> ETGQVAASPSINVALKAAFPSPPYLVELLETAASDNTTIYYSLLDRIAKGHFAEATTDKALYEKFLEVLRDDGHMDPEALSAFKLALSLRTATPRVEAHYQYYTATVEPSLSGTQEGCDQWFLIDGEQYCSPTLDTSHGKVKGEDQLRTLPFDRKFGVGSRDVILYADITSKSFAPFHEVAMDLAKKGKASYRVRYRRSPSHSRESLSVNGYGVELVLKRTDYIVIDDRDTGAAAKPAEENDQKPLVGHETVLDDGEEIADIKPLEKSELAALGMKAASFVMQSEKPFEALLKLTQDFPKYSNSLGSQNVSAEFEAEHRGNREVFLPEGSNVLWLNGLHLIDRQIQPFGLVDLLTRERKLIKSVLDLGLTGQQAVDLLGHAEVAHAKSGDDEPRRFDWRDDIEEGQVIIWLNNLEKDKRYKSFSPSIWVLIHHFGHGLPQIRRDVFNLVVPVDLTKADDVKIVVEGLLSFVKRLIPVRFGFVPLTPTGQAIDQAKVVYYLLENYGLAAATAYLEKSYEEQSTGQPNERIFNEVIKDKSLRPDGVELSFKDIFISEKHEKQIHLSKHWVERLRAGGDVPTVFFDGFPIPREDNWLRVMNHRLMQDLQALQQAGYFGMLNESMWLPGFFLEKALSRRNTLIFPEDKNELTVLNVNKIYIENHDLMSKVPVIEASKESTRDDWAALTVVADLDDIEGQELVYYALRFRKSNDGVRLDIVHNPKDTSRSPSVLAQRLKSREDKLLDFTRFLDLETALETGEFEPDVAYDASLANFLASSNMKAGDNFVILNGRVLGPITSADDFKKEDFEVFLQAERRTRILPVYKALEDLGLDDKVSGPLSAAKLTSVT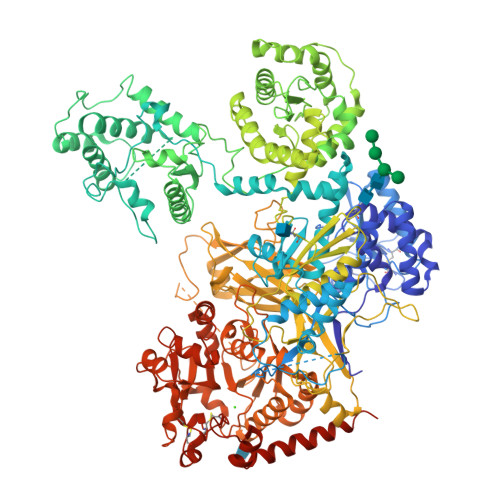ALSTISDLPQGIFDNAPTVRTTLFKQWNSTYTSFEVGDASTATIFFVAVINPASEIGQRWVAVLKVLSELEGVHLRVFLNPTVMIEELPVKRFYRYVLSSSPSFDESGKVKALSARFTGVPRETLLVVGMDVPPAWLVTSKVAVDDLDNLRIKDIKAKRGTEHVEAIYELEHILIEGHSREIPGAHAPRGVQLVLETENNPHFADTIIMANLGYFQFKANPGVYNIRLKEGRSSEIFTLESVGAKGWGPIPGDDNTEVVLMDFQGTTLYPRLRRKPGMEEEDVLEPSTKSGEESGSGARNLVSRGIKFAEGLLGRGNKAAEATKSVSKTEHAEINIFSVASGHLYERMLNIMMASVMHHTNHTVKFWFIEQFLSPSFKDFIPHMAAEYGFKYEMVTYKWPHWLRQQKEKQREIWGYKILFLDVLFPLSLDKVIFVDADQIVRTDMYDLVEHPLDGAPYGFAPMCDSRVEMEGYRFWKTGYWANYLKGKPYHISALYVVDLQRFRELAAGDRLRQQYHALSADPNSLANLDQDLPNHMQFTIPIATLPQEWLWCETWCSDETLKDARTIDLCNNPMTKEPKLDRARRQVPEWTKYDEEIAELARRVREEKPKKKEEEKVQKNPKSRRLDGDEEEVKTVREGTKHHHHHH> GSHMETAKEPCMAKFGPLPSKWQMASSEPPCVNKVSDWKLEILQNGLYLIYGQVAPNAAYNDVAPFEVRLYKNKDMIQTLTNKSKIQNVGGTYELHVGDTIDLIF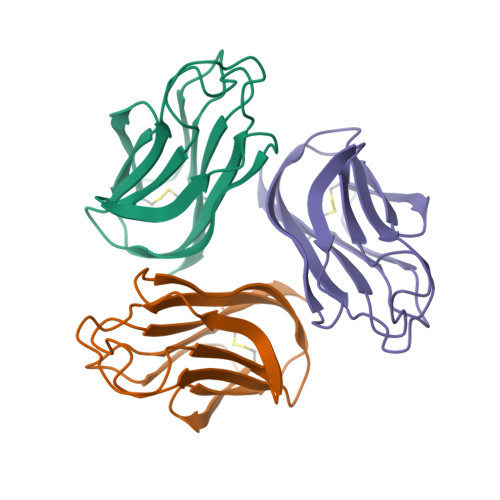NSEHQVLKNNTYWGIILLANPQFIS>GPLHMRKGYKVLAIETSCDDTCVSVLDRFSKSAAPNVLANLKDTLDSIDEGGIIPTKAHIHHQARIGPLTERALIESNAREGIDLICVTRGPGMPGSLSGGLDFAKGLAVAWNKPLIGVHHMLGHLLIPRMGTNGKVPQFPFVSLLVSGGHTTFVLSRAIDDHEILCDTIDIAVGDSLDKCGRELGFKGTMIAREMEKFINQDINDQDFALKLEMPSPLKNSASKRNMLSFSFSAFITALRTNLTKLGKTEIQELPEREIRSIAYQVQ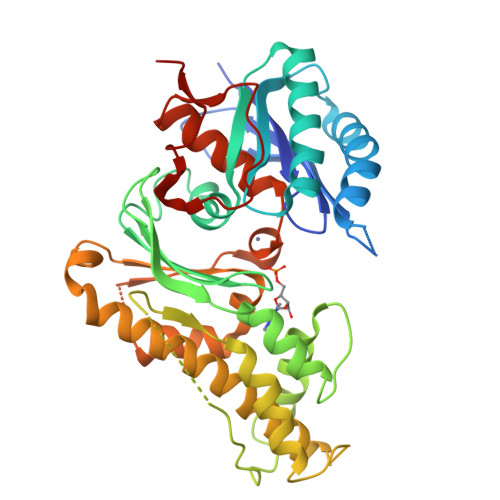ESVFDHIINKLKHVLKSQPEKFKNVREFVCSGGVSSNQRLRTKLETELGTLNSTSFFNFYYPPMDLCSDNSIMIGWAGIEIWESLRLVSDLDICPIRQWPLNDLLSVDGWRTDQL[2x]> MANVWGVRLADSLSSPTIETRTRQYTLHDLCSDLDANPGREPWKPLRNQRTNNIVAVQLFRPLQGLVLDTQLYGFPGAFDDWERFMREKLRVLKYEVLRIYPISNYSNEHVNVFVANALVGAFLSNQAFYDLLPLLIINDTMIGDLLGTGASLSQFFQSHGDVLEVAAGRKYLQMENYSNDDDDPPLFAKDLSDYAKAFYSDTYEVLDRFFWTHDSSAGVL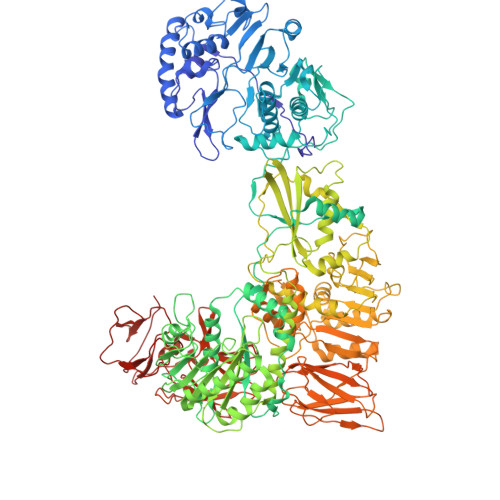VHYDKPTNGHHYLLGTLTQMVSAPPYIINATDAMLLESCLEQFSANVRARPAQPVTRLDQCYHLRWGAQYVGEDSLTYRLGVLSLLATNGYQLARPIPRQLTNRWLSSFVSQIMSDGVNETPLWPQERYVQIAYDSPSVVDGATQYGYVRKNQLRLGMRISALQSLSDTPSPVQWLPQYTIDQAAMDEGDLMVSRLTQLPLRPDYGNIWVGDALSYYVDYNRSHRVVLSSELPQLPDTYFDGDEQYGRSLFSLARKIGDRSLVKDTAVLKHAYQAIDPNTGKEYLRSGQSVAYFGASAGHSGADQPLVIEPWIQGKISGVPPPSSVRQFGYDVARGAIVDLARPFPSGDYQFVYSDVDQVVDGHDDLSISSGLVESLLSSCMHATAPGGSFVVKINFPTRPVWHYIEQKILPNITSYMLIKPFVTNNVELFFVAFGVHQHSSLTWTSGVYFFLVDHFYRYETLSTISRQLPSFGYVDDGSSVTGIETISIENPGFSNMTQAARIGISGLCANVGNARKSIAIYESHGARVLTITSRRSPASARRKSRLRYLPLIDPRSLEVQARTILPADPVLFENVSGASPHVCLTMMYNFEVSSAVYDGDVVLDLGTGPEAKILELIPATSPVTCVDIRPTAQPSGCWNVRTTFLELDYLSDGWITGVRGDIVTCMLSLGAAAAGKSMTFDAAFQQLIKVLSKSTANVVLVQVNCPTDVVRSIKGYLEIDSTNKRYRFPKFGRDEPYSDMDALEKICRTAWPNCSITWVPLSYDLRWTRLALLESTTLSSASIRIAELMYKYMPIMRIDIHGLPMEKRGNFIVGQNCSLVIPGFNAQDVFNCYFNSALAFSTEDVNAAMIPQVSAQFDATKGEWTLDMVFSDAGIYTMQALVGSNANPVSLGSFVVDSPDVDITDAWPAQLDFTIAGTDVDITVNPYYRLMTFVRIDGQWQIANPDKFQFFSSASGTLVMNVKLDIADKYLLYYIRDVQSRDVGFYIQHPLQLLNTITLPTNEDLFLSAPDMREWAVKESGNTICILNSQGFVLPQDWDVLTDTISWSPSIPTYIVPPGDYTLTPL>[3x]GSHMGQSLRTLQGHQ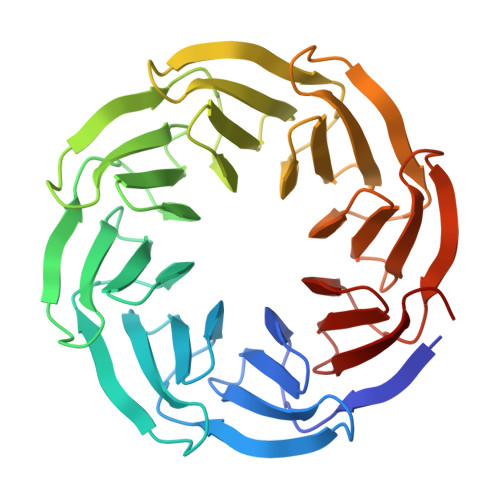SAVTSLQFNDNIVVSGSDDSTVKVWDIKTGQSLRTLQGHQSAVTSLQFNDNIVVSGSDDSTVKVWDIKTGQSLRTLQGHQSAVTSLQFNDNIVVSGSDDSTVKVWDIKTGQSLRTLQGHQSAVTSLQFNDNIVVSGSDDSTVKVWDIKTGQSLRTLQGHQSAVTSLQFNDNIVVSGSDDSTVKVWDIKTGQSLRTLQGHQSAVTSLQFNDNIVVSGSDDSTVKVWDIKTGQSLRTLQGHQSAVTSLQFNDNIVVSGSDDSTVKVWDIKTGQSLRTLQGHQSAVTSLQFNDNIVVSGSDDSTVKVWDIKGS>[8x]MLIQHVQ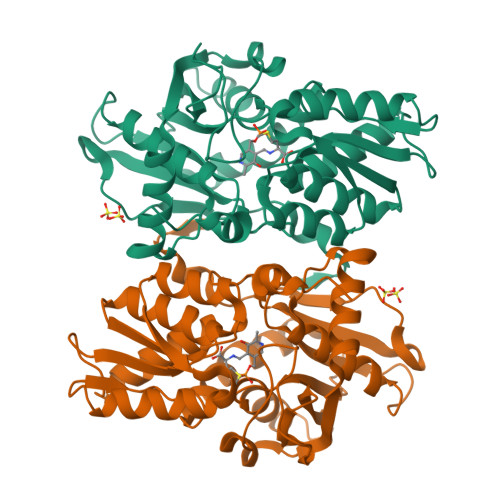ELIGHTPLMALPIEVPNHSHIYAKLEMFNPGGSIADRLGAYLIEDGLQRGRVNAKTTIIEPTAGNTGIGLALATQAHHLRTILVVPEKFSMEKQVLMQALGAEIVHTPSEEGIKGAIRKAEALAATISNSYVPMQFKNPANPAAYYHTLAPEILADMPAPITAFVAGAGSGGTFAGVAAYLQAQDSATKAVVVEPEGSILNGGPAHAHRTEGIGVEFIPPFFDQVRIDQTLTIADNDAFAQVRHLARDHGLLIGSSSGAALAASLQLATNLPANSHIVTIFPDSSERYLSQKIYTKLEHHHHHH>GAMGPTSNDACLSIVHSLMCHRQGGESETFAKRAIESLVKKLKEKKDELDSLITAITTNGAHPSKCVTIQRTLDGRLQVAGRKGFPHVIYARLWRWPDLHKNELKHVKYCQYAFDLKCDSVCVNPYHYERVVSPG[2x]

Smad proteins consist of an N-terminal MH1 domain, which binds to DNA, a linker region with phosphorylation sites for network regulatory inputs, and a C-terminal MH2 domain that is phosphorylated by the receptors and binds other Smad proteins, LDTFs, chromatin readers, and transcriptional co-activators and co-repressors. The receptors for TGF-β, nodal, activin, myostatin, and other family members are membrane serine/threonine kinases that phosphorylate and activate Smad2 and Smad3, whereas analogous receptors for the bone morphogenetic proteins (BMPs) preferentially phosphorylate and activate Smads 1, 5, and 8. These receptor-activated Smads (R-Smads) form heterotrimeric complexes with Smad4, which is required for the transcriptional regulation of most target genes. Focusing on the human and mouse Gsc promoter, here we identify specific Smad-binding GC-rich motifs and provide the X-ray crystal structures of Smad3 and Smad4 bound to several of these motifs. The structures determined here reveal that the β-hairpin is flexible and adaptable to bind with high-affinity several variants of the consensus sequence GGC(GC)|(CG), which we refer to as 5GC SBE.

The GC-rich region of Gsc contains a conserved GGCTG sequence, which resembles the GTCT-AGAC SBE. We determined how the T to G change modified the recognition of the motif by Smad3 and Smad4 using a palindromic version of the motif similar to the canonical SBE. The X-ray crystal structure of the Smad4 MH1 domain in complex with a GGCT-AGCC oligonucleotide was determined at 2.98 Å resolution (space group P212121). The ASU contains two Smad4 MH1 monomers and one dsDNA molecule. Contacts were detected from Arg81 to G5 in one DNA strand and from Gln83 to A9′ in the complementary DNA strand. The conformation of the Smad-bound GGCT motif is intermediate between that of GTCT and that of GGCGC. We analyzed the superposition of the Smad4 MH1 domain bound to different DNAs with Cα root mean square deviations (RMSD) of 0.47 Å and of 0.45 Å for the GTCT and GGCT, respectively, for 114 aligned residues.> MTAFGVEPYGQPKYLEIAGKRMAYIDEGKGDAIVFQHGNPTSSYLWRNIMPHLEGLGRLVACDLIGMGASDKLSPSGPDRYSYGEQRDFLFALWDALDLGDHVVLVLHDWGSALGFDWANQH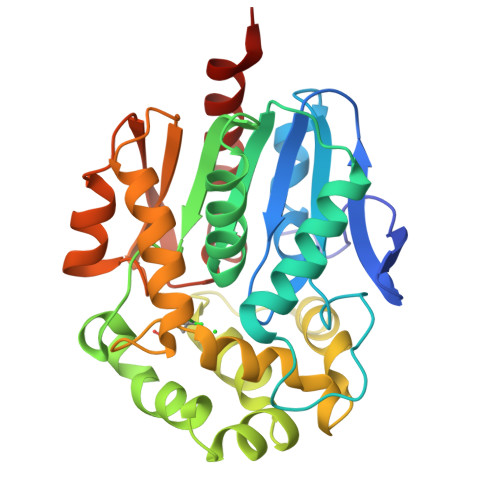RDRVQGIAFMEAIVTPMTWADWPPAVRGVFQGFRSPQGEPMALEHNIFVERVLPGAILRQLSDEEMNHYRRPFVNGGEDRRPTLSWPRNLPIDGEPAEVVALVNEYRSWLEETDMPKLFINAEPGAIITGRIRDYVRSWPNQTEITVPGVHFVQEDSPEEIGAAIAQFVRRLRSAAGV> MLATPFYSRSDRIFGIVNAVLLGIFALCALYPIIYIFSMSISSGAAVTQGRVFLLPVDIDFSAYGRVLHDKLFWTSYANTIFYTVFGVVTSLIFIVPGAYALSKPRIRGRRVFGFIIAFTMWFNAGMIPFFLNMRDLGLLDNRFGILIGFACNAFNIILMRNYFESISASFEEAARMDGANDLQILWKVYIPLAKPALATITLLCAISRWNGYFWAMVLLRAEEKIPLQVYL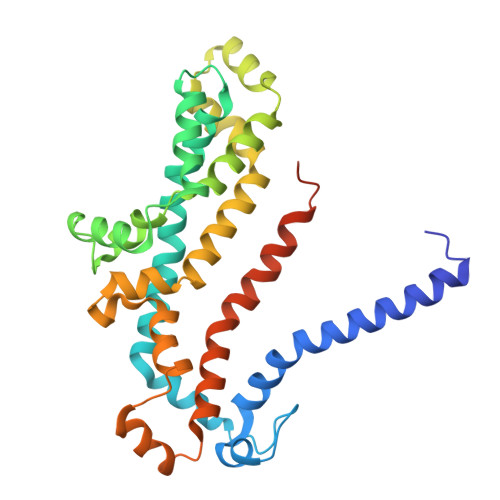KKTIVDLNVNEEFAGALLTNSYSMETVVGAIIVMSIIPVIIVYPVVQKYFTKGVMLGGVKELEHHHHHHHHHH> MFQTFISRHNSNFFSDKLVATSVTPASLAPVLQTPKAASSTLYFNQLTVNAGNGGFLHCIQMDTSVNAANQVVSVGADIAFDADPKFFACLVRFESASVPTTLPTDYDVYPLDGRHDGGYYTVKDCVTIDVLPREPGNNVYVGFMVWSNFTATKCRG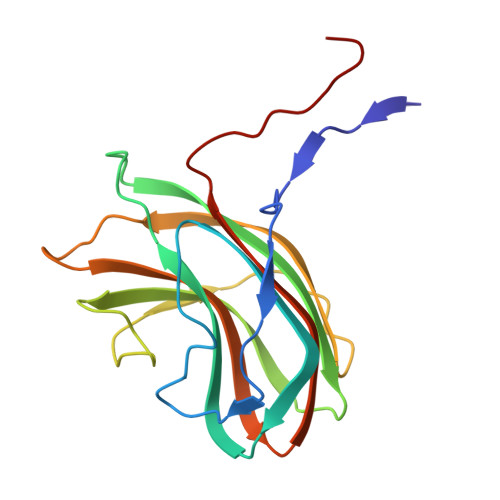LVSLNQVIKEIICLQPLK>MHHHHHHTTTPTVTVLGLGPMGQALSRALLDAGHTVTVWNRTESKAQALRDRGALSAPTPAAAIAASDLALVNVVDHDAVDAILTAAGDAPAGRTVIGLSSDTPDRARRTAKLVGNVGGRYLDGAIMTPIDTIGTRGASILFAGPQALFDEHRGVLDTLGQLTWVGEDHGRAAAFDMALLDLFWTSVGGFGHALMVARANGIEPSELMPHAHGIVGILSPIFTEVAQRVEDDRHSDASASVSSVASSVRHLIAASREAGVDAGLLEAFRGYVDATVAAGHGDDEISRIASEMTTLTRG[5x]

In the early 2010s, Mitsukura et al. discovered, purified and characterized NADPH-dependent imine reductases (IREDs) from Streptomyces strains, a new enzyme class capable of the conversion of heterocyclic prochiral imines to chiral amines with high enantioselectivity. Crystallographic studies so far indicate a close similarity in the overall structure of these enzymes. They consist of an N-terminal Rossmann-fold and a C-terminal helical domain, connected by a long interdomain helix, and constitute a catalytically active dimer by reciprocal domain sharing. Out of all the IREDs we tested, the S-enantioselective IRED from Mycobacterium smegmatis (S-IRED-Ms), a member of the IRED superfamily 3 (SFam3) first characterized by Wetzl et al. in 2015, proved to be the only one capable of reducing both 3-thiazolines and 2H-1,4-benzothiazines with promising activity and excellent enantioselectivity. In order to further elucidate this, we present a high-resolution crystal structure of S-IRED-Ms together with its cofactor NADPH, the first published structure of an SFam3 IRED.

The S-IRED-Ms monomer, represented by subunit A, consists of an N-terminal Rossmann-fold domain of 160 amino acids (9–169) and a C-terminal helical domain (201–294) connected by a long interdomain helix (170–200). The dimers are generated by reciprocal domain swapping, where the end of N-terminal domain A, the interdomain helix α7 protrudes and inserts through a hydrophobic channel in the C-terminal domain of chain B to then emerge and continue as the C-terminal helical domain of A, which contacts the N-terminal domain of subunit B. The cleft formed between the Rossmann-fold domain of subunit A and the helical domain of subunit B constitutes the active site of S-IRED-Ms and is a large channel at the dimer interface with two separate openings, presumably for individual binding of NADPH and a substrate, respectively. The electron density obtained after molecular replacement allowed for unequivocal placement of five NADPH molecules in the asymmetric unit, one in each S-IRED-Ms monomer active site. Apart from hydrogen bonds to S232 and S237, NADPH only interacts with the N-terminal domain. The nicotinamide ring is held in place by interactions with S232 and stacks against M15 with its si-face presented to the presumed substrate-binding area of the active site. The second entrance to the active site in S-IRED-Ms, situated between the loop connecting the β-strands β6 and β7 of one S-IRED-Ms monomer and the loop connecting α-helices α8 and α9 as well as helix α8 itself of the other monomer is characterized by a strongly negative electrostatic surface potential, largely due to D125, E218 and possibly to a lesser extent P214 and S232 outlining the entrance.> GSHMFYFLSKRRRNLLRNPCGEEDLEGWSDVEHGGDGWKVEELPGDGNVEFTQDDSVKKYFASSFEWCRKAQVIDLQAEGYWEELLDTTQPAIVVKDWYSGRTDAGSLYELTVRLL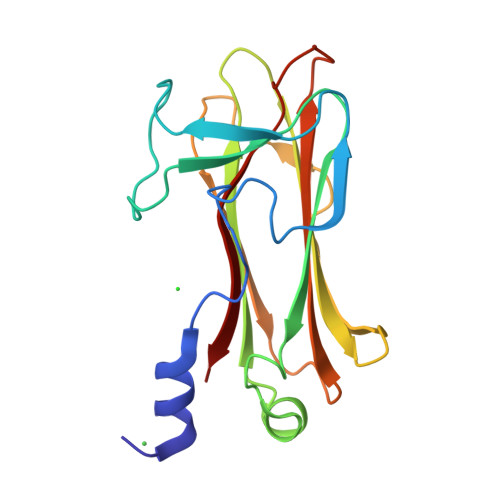SENEDVLAEFATGQVAVPEDGSWMEISHTFIDYGPGVRFVRFEHGGQDSVYWKGWFGARVTNSSVWVEP>[2x]GSHMGRGAFLSRHSLDMKFTYCDDRIAEVAGYSPDDLIGCSAYEYIHALDSDAVSKSIHTLLSKGQAVTGQYRFLARSGGYLWTQTQATVVSGGRGPQSESIVCVHFLISQVEET

HIF, closely linked to disorders of the circulatory system and cancer progression, consists of two multidomain subunits including the constitutively expressed HIF-1β and an oxygen-labile HIF-1α (or paralogs HIF-2α and -3α). HIF-3α9, the longest (669 aa) and canonical isoform3, is a potent oxygen-labile transcription factor, tightly regulating the expression of a unique set of genes. Due to the use of different transcription initiation sites and a combination of splicing events in HIF3A, the C-terminal Per-Arnt-Sim sensor domain (PASb) is the only common architectural feature among the HIF-3α isoforms. The PASb domains in both HIF-α and -β subunits have a crucial role in forming active HIF heterodimers and recruiting co-regulators.

Hereby, we present the crystal structure of the recombinant human HIF-3α PASb, or PASb-3α, at 1.15 Å maximum resolution. Although with a backbone virtually identical to that of the PASb domains of both HIF-1α9 and HIF-2α10, PASb-3α has a unique extensive C-shaped hydrophobic cavity of 510 Å3. We identified a 1-(11Z-octadecenoyl)-sn-glycerol molecule of bacterial nature buried in this cavity, as clearly suggested by the size and geometrical features of the electron density map. As such, the aliphatic tail of the fatty acid extended to eighteen carbons in length (maximum length limited by the cavity size), with a cis double bond between C11 and C12, interspersed by four gauche configurations (at positions C5, C7, C9 and C13,). The ester group at the glycerol sn-1 position makes polar contact with the main chain carboxyl group of His339 and main chain amino group of Leu340. The sn-2 position is not substituted, also sharing a hydrogen bond with the Leu340 main chain amino group. Based solely on the electron density map, we could not tell whether the glycerol sn-3 position was substituted, due to absence of well-structured atoms beyond its remaining hydroxyl group. However, the presence of a well-coordinate sulfate ion (abundant in the crystallization solution), 6 Å apart from the glycerol sn-3 hydroxyl, suggested that PASb-3α could also bind to phospholipids. Collectively, all complex lipids identified as PASb-3α ligands include the 18-carbon unsaturated 11Z-octadecenoic acid (or cis-vaccenic acid; 18:1, cis-11) and an unmodified sn-2 glycerol position as common structural denominators. For the first time, we document that a eukaryotic PAS domain may have lipids as high-affinity cofactors, thus introducing a new class of PAS ligands and expanding its already vast functional portfolio.>[4x]ARKCSLTGKWTNDLGSNMTIGAVNSRGEFTGTYITAVTATSNEIKESPLHGTQNTINKRTQPTFGFTVNWKFSESTTVFTGQCFIDRNG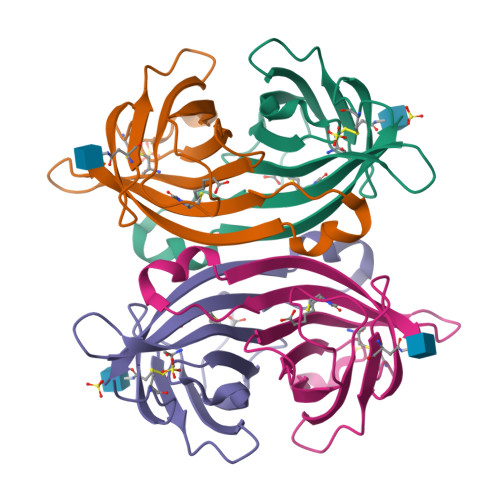KEVLKTMWLLRSSVNDIGDDWKATRVGINIFTRL> GSPLQDNLVIALHSYEPSHDGDLGFEKGEQLRILEQSGEWWKAQSLTTGQEGFIPFNFV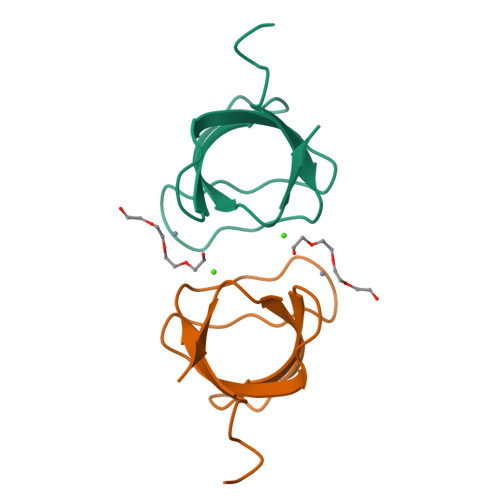AKA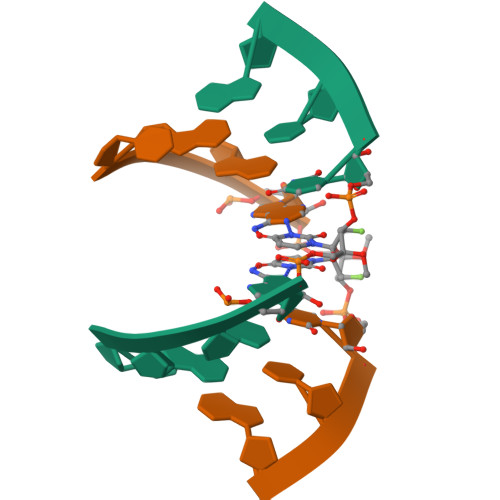>[4x]CGAAXUCG> MFENITAAPADPILGLADLFRADERPGKINLGIGVYKDETGKTPVLTSVKKAEQYLLENETTKNYLGIDGIPEFGRCTQELLFGKGSALINDKRARTAQTPGGTGALRVAADFL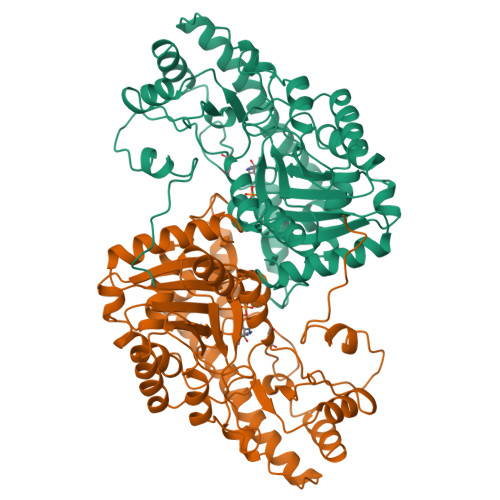AKNTSVKRVWVSNPSWPNHKSVFNSAGLEVREYAYYDAENHTLDFDALINSLNEAQAGDVVLFHGSCHNPTGIDPTLEQWQTLAQLSVEKGWLPLFDFAYQGFARGLEEDAEGLRAFAAMHKELIVASSYSKNFGLYNERVGACTLVAADSETVDRAFSQMKAAIRANYSNPPAHGASVVATILSNDALRAIWEQELTDMRQRIQRMRQLFVNTLQEKGANRDFSFIIKQNGMFSFSGLTKEQVLRLREEFGVYAVASGRVNVAGMTPDNMAPLCEAIVAVL>MMELIRIAMKKDLENDNSLMNKWATVAGLKNPNPLYDFLNHDGKTFNEFSSIVNIVKSQYPDREYELMKDYCLNLDVKTKAARSALEYADANMFFEIEDVLIDSMISCSNMKSKEYGKVYKIHRELSNSVITEFEAVKRLGKLNIKTPEMNSFSRLLLLYHYLSTGNFSPMAQLIKQIDLSEISENMYIRNTYQTRVHVLMSNIKLNENSLEECREYSKKALESTNILRFQVFSYLTIGNSLLFSNYELAQENFLKGLSISVQNENYNMIFQQALCFLNNVWRKENKWINFESDSIMDLQEQAHCFINFNENSKAKEVLDKLDLLVHNDNELAMHYYLKGRLEQNKACFYSSIEYFKKSNDKFLIRLPLLELQKMGENQKLLELLLLLEHHHHHH[2x]

Recently, in Bacillus phages, a peptide communication system named the arbitrium system was identified that plays an essential role in lysis–lysogeny decisions during infection of Bacillus host cells. This system requires the arbitrium hexapeptide to bind to its cellular receptor AimR to regulate transcription of the lysogeny negative regulator gene aimX. AimR is composed of two domains, a N-terminal domain that is responsible for DNA binding and a C-terminal domain that specifically recognizes the arbitrium peptide. The overall structure of AimR is similar to that of RRNPP family proteins.

In our previous reported structures of apo- and peptide-bound AimR, we were unable to trace the N-terminal DBD structure due to the poor electronic densities. In this study, we reoptimized the crystals and collected new datasets for AimR with or without the peptide. Finally, we traced the density of the DBD for AimR with or without the peptide. Here, we updated the apo- and peptide-bound form structures containing the DBD, although there were only subtle differences between them. In the apo- and peptide-bound form, the AimR dimer exhibits an inverted trapezoid-like fold. The last C-terminal capping helices from two AimR molecules undergo dimerization via a network of van der Waals interactions. The distance between the two aspartic acid residues in the inner cavity, D15 of AimRA and D15 of AimRB, is approximately 125 Å in apo- or peptide-bound AimR. The low- and high-FRET efficiencies are centered at 30% and 60%, with respective populations of ~43% and ~57%. Hence, in solution, AimR alone exists in two dynamic conformational states that correspond to the open and closed conformations according to the low- and high-FRET efficiencies. In the absence of the arbitrium peptide, dimeric AimR exhibits the dynamic open and closed conformations equally, which favor peptide and DNA binding, respectively.>QFTDSCLRCICKVEGCDSQIGKCGMDVGSLSCGPYQIKKPYWIDCGKPGGGYESCTKNKACSETCVRAYMKRYGTFCTGGRTPTCQDYARIHNGGPRGCKSSATVGYWNKVQKCLRGTHHHHHH[2x]

Destabilase from the medical leech Hirudo medicinalis belongs to the family of i-type lysozymes. It has two different enzymatic activities: microbial cell walls destruction (muramidase activity), and dissolution of the stabilized fibrin (isopeptidase activity). The main difference between low and high salt structures as well as between the two chains of high salt structure is tied to a flexible loop (Gly44-Ser51), containing enzymatically important Asp46. Together with Glu34, Asp46 forms a catalytic dyad for muramidase activity in i-type lysozymes.

To get structural insights into destabilase function we solved its structure in two different crystal forms: P1—obtained at pH 5.0 and high sodium salt concentrations (2.9 M sodium malonate) and P21—obtained at pH 8.0 and low sodium concentration (0.3 M sodium chloride). In the high salt structure, both protein chains possess a more compact Gly44-Ser51 loop adherent to the protein core. Asp46 has two alternative conformations in both chains and in all cases is oriented towards Glu34. In our high salt structure, both A and B chains contain one sodium ion with 50% occupancy situated in the cleft between Glu34 and Asp46 and stabilized in octahedral coordination with water molecules by Glu34 and Asp46 side chains. Remarkably, in addition to its high sodium content, the crystallization sample of the high salt destabilase structure also included a muramidase product inhibitor NAG3. However, electron density maps did not reveal the presence of NAG3 molecule, suggesting that the inhibitory effect of sodium ions was at play. Given that the sodium ion appears near Ser51 in our high salt structure, we propose this serine to be the nucleophile in destabilase.> MSSMILTQFGPFIESISGITDQSNDVFEDAAKAFSMFTRSDVYKALDEIPFSDDAMLPIPPTIYTKPSHDSYYYIDALNRVRRKTYQGPDDVYVPNCSIVELLEPHETLTSYGRLSEAIENRAKDGDSQARIATTYGRIAESQARQIKAPLEKFVLALLVAEAGGSLYDPVLQKYDEIPDLSHNCPLWCFREICRHISGPLPDRAPYLYLSAGVFWLMSPRMTSAIPPLLSDL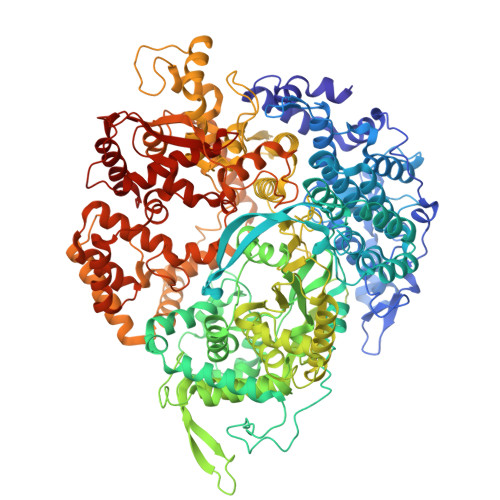VNLAILQQTAGLDPSLVKLGVQICLHAAASSSYAWFILKTKSIFPQNTLHSMYESLEGGYCPNLEWLEPRSDYKFMYMGVMPLSAKYARSAPSNDKKARELGEKYGLSSVVGELRKRTKTYVKHDFASVRYIRDAMACTSGIFLVRTPTETVLQEYTQSPEIKVPIPQKDWTGPIGEIRILKDTTSSIARYLYRTWYLAAARMAAQPRTWDPLFQAIMRSQYVTARGGSGAALRESLYAINVSLPDFKGLPVKAATKIFQAAQLANLPFSHTSVAILADTSMGLRNQVQRRPRSIMPLNVPQQQVSAPHTLTADYINYHMNLSTTSGSAVIEKVIPLGVYASSPPNQSINIDISACDASITWDFFLSVIMAAIHEGVASSSIGKPFMGVPASIVNDESVVGVRAARPISGMQNMIQHLSKLYKRGFSYRVNDSFSPGNDFTHMTTTFPSGSTATSTEHTANNSTMMETFLTVWGPEHTDDPDVLRLMKSLTIQRNYVCQGDDGLMIIDGTTAGKVNSETIQKMLELISKYGEEFGWKYDIAYDGTAEYLKLYFIFGCRIPNLSRHPIVGKERANSSAEEPWPAILDQIMGVFFNGVHDGLQWQRWIRYSWALCCAFSRQRTMIGESVGYLQYPMWSFVYWGLPLVKAFGSDPWIFSWYMPTGDLGMYSWISLIRPLMTRWMVANGYVTDRCSPVFGNADYRRCFNELKLYQGYYMAQLPRNPKKSGRAAPREVREQFTQALSDYLMQNPELKSRVLRGRSEWEKYGAGIIHNPPSLFDVPHKWYQGAQEAAIATREELAEMDETLMRARRHSYSSFSKLLEAYLLVKWRMCEAREPSVDLRLPLCAGIDPLNSDPFLKMVSVGPMLQSTRKYFAQTLFMAKTVSGLDVNAIDSALLRLRTLGADKKALTAQLLMVGLQESEADALAGKIMLQDVNTVQLARVVNLAVPDTWMSLDFDSMFKHHVKLLPKDGRHLNTDIPPRMGWLRAILRFLGAGMVMTATGVAVDIYLEDIHGGGRSLGQRFMTWMRQEGRSA> MRGRLQGVELIARDWIGLMVEVVESPNHS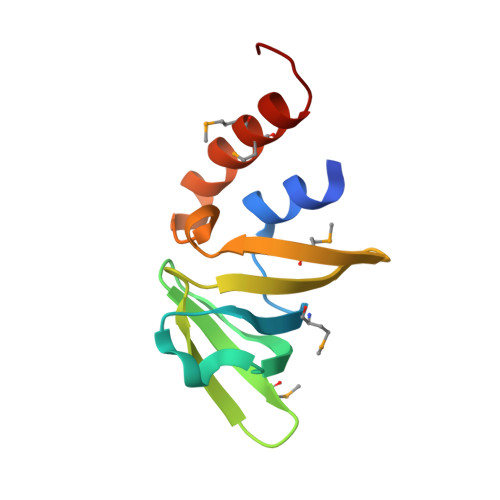EVGIKGEVVDETQNTLKIMTEKGLKVVAKRGRTFRVWYKGKIMRIKGDLINFRPEDRIKRGLMMLKRAKGVWI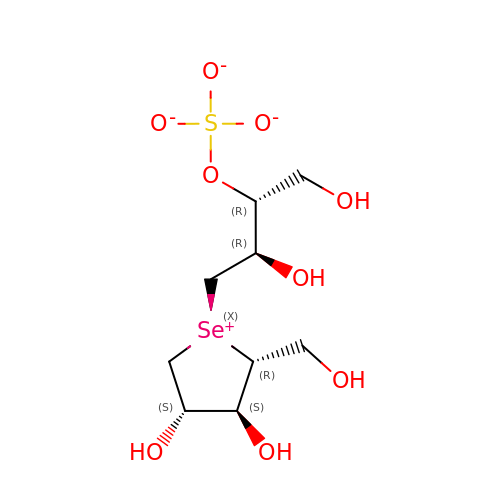1,4-DIDEOXY-1,4-[[2R,3R)-2,4-DIHYDROXY-3-(SULFOXY)BUTYL]EPISELENONIUMYLIDENE]-D-ARABINITOL INNER SALT | C9 H18 O9 S Se | WLNWUNIGATZIKW-KNCZUUIASA-L> AVSDQRLSEATLRELEDERQRAGL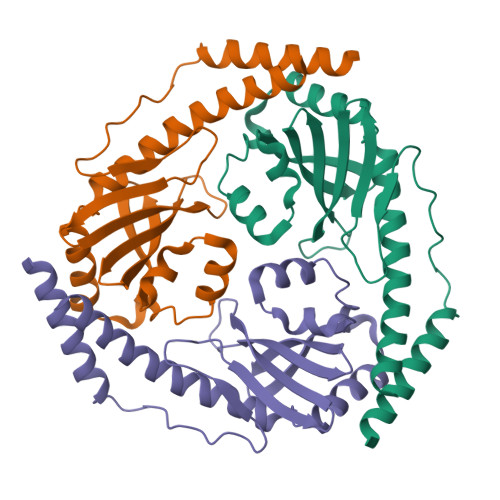PEKPEIPEGWTIDRKPGVTHFTMRKSHGDEEIILQLTGEDRSNEEITRTLDVLVVNGGKALVFGMSVEDGEFVINNVCFRHDGKLALDTSAEAQFQKSQLYMGPDLADLEDHLVDSFTSYLSARGVNDTLANFIDQFSLWSEQADYEEWLSSINKFVS>GTKQEKTALNMARFIRSQTLTLLEKLNELG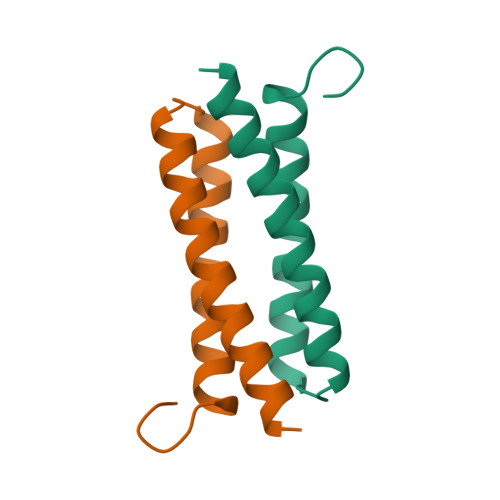ADEQADICESLHDHADELYRSCLARFGDDGEN[3x]> AAKMAFTLADRVTEEMLADKAALVVEVVEENYHDAPIVGIAVVNEHGRFFLRPETALADPQFVAWLGDETKKKSMFDSKRAAVALKWKGIELCGVSFDLLLAAYLLDPAQGVDDVAAAAKMKQYEAVRPDEAVYGKGAKRAVPDEPVLAEHLVRKAAAIWALERPFLDELRRNEQDRLLVELEQPLSSILAEMEFAGVKVDTKRLEQMGEELAEQLRTVEQRIYELAGQEFNINSPKQLGVILFEKLQLPVLKKSKTGYSTSADVLEKLAPYHEIVENILHYRQLGKLQSTYIEGLLKVVRPDTKKVHTIFNQALTQTGRLSSTEPNLQNIPIRLEEGRKIRQAFVPSESDWLIFAADYSQIELRVLAHIAEDDNLMEAFRRDLDIHTKTAMDIFQVSEDEVTPNMRRQAKAVNFGIVYGISDYGLAQNLNISRKEAAEFIERYFESFPGVKRYMENIVQEAKQKGYVTTLLHRRRYLPDITSRNFNVRSFAERMAMNTPIQGSAADIIK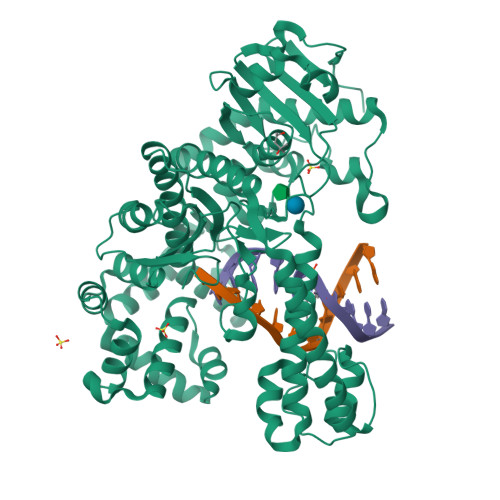KAMIDLNARLKEERLQARLLLQVHDELILEAPKEEMERLCRLVPEVMEQAVTLRVPLKVDYHYGSTWYDAK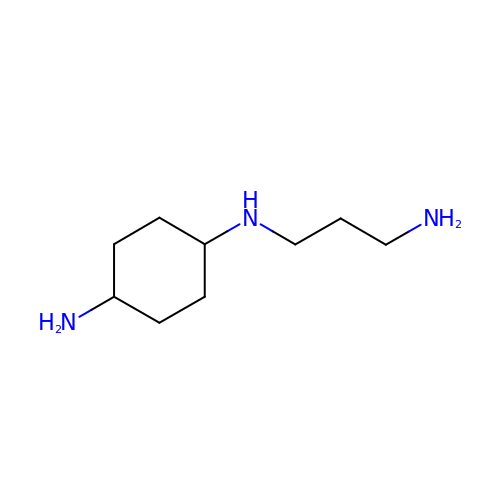trans-N-(3-aminopropyl)cyclohexane-1,4-diamine | C9 H21 N3 | QIMPCSMJRMPRJC-KYZUINATSA-N> MLTEGISIQSYD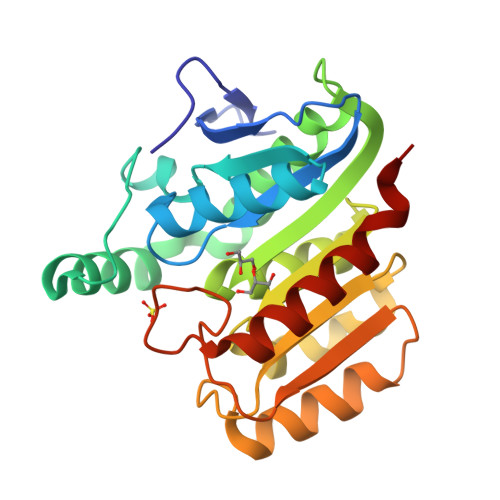GHTFGALVGSPAKAPAPVIVIAQEIFGVNAFMRETVSWLVDQGYAAVCPDLYARQAPGTALDPQDERQREQAYKLWQAFDMEAGVGDLEAAIRYARHQPYSNGKVGLVGYSLGGALAFLVAAKGYVDRAVGYYGVGLEKQLNKVPEVKHPALFHMGGQDHFVPAPSRQLITEGFGANPLLQVHWYEEAGHSFAATSSSGYVASAAALANERTLDFLAPLQSKKP Curli are functional amyloids that play critical roles in biofilm formation and adhesion in many Enterobacteriaceae. Two outer membrane proteins, CsgG and CsgF, form the core apparatus for secretion and assembly of the curli structural subunits. In this work, we show that CsgF forms a stable complex with CsgG via a 1:1 stoichiometry by lining the extracellularly faced lumen of the nonameric CsgG channel via its N-terminal 27 residues, creating a secretion channel with 2 constriction regions for curli subunit secretion. The free C-terminal domain of CsgF recruits and binds the secreted nucleator CsgB, creating a growth point for further addition of CsgA subunits.

To improve the resolution of the cryo-EM structure of the CsgG-CsgF complex in order to accurately locate side chains of 9 Asn36 residues of CsgF that consist of the upper constriction region of the CsgG-CsgF channel, the purified CsgG-CsgF complex was proteolytically digested with chymotrypsin to remove flexible regions of the CsgG-CsgF complex that may affect the stability of the complex in the detergent-containing buffers and increase particle heterogeneity on the grid. The resulted protein sample (denoted as the CsgG-CsgF20–59 complex) contained a variant of CsgG that includes residues 47–252 in complex with the most N-terminal 40 residues of the mature CsgF (CsgF20–59), as confirmed by mass spectrometric analysis. In contrast to the oligomerization state exhibited on size exclusion chromatography, the CsgG-CsgF20–59 complexes tended to form filaments with varied lengths on the cryo-EM grids. Using a similar cryo-EM structure determination approach we obtained 2 maps for the nonameric CsgG-CsgF20–53 complex and the nonameric CsgG-CsgF20–59 complex, with an overall resolution of 2.9 Å and 3.2 Å, respectively (S4C, S4D). As expected, the 2.9-Å cryo-EM map of the CsgG-CsgF20–53 complex allows us to ascertain all the side chains of CsgF20–53 unambiguously—in particular side chains of the 9 Asn36 residues that consist of the upper constriction region of the CsgG-CsgF channel (right).

>MQRLFLLVAVMLLSGCLTAPPKEAARPTLMPRAQSYKDLTHLPAPTGKIFVSVYNIQDETGQFKPYPASNFSTAVPQSATAMLVTALKDSRWFIPLERQGLQNLLNERKIIRAAQENGTVAINNRIPLQSLTAANIMVEGSIIGYESNVKSGGVGARYFGIGADTQYQLDQIAVNLRVVNVSTGEILSSVNTSKTILSYEVQAGVFRFIDYQRLLEGEVGYTSNEPVMLCLMSAIETGVIFLINDGIDRGLWDLQNKAERQNDILVKYRHMSVPPESWSHPQFEK[9x];>[9x]MRVKHAVVLLMLISPLSWAGTMTFQFRNPNFGGNPNNGAFLLNSAQAQNSYKDPSYNDDFGIETPSALDNFTQAIQSQILGGLLSNINTGKPGRMVTNDYIVDIANRDGQLQLNVTDRKTGQTSTIQVSGLQNNSTDFHHHHHH>MRGSHHHHHHGSTEISLEGLHRNMGEQLFDGDILATGRIICRERHTGFHIQMNARQVEGRPGHYIVQGSKDTQSKLWVRLGREGWTSPTGGGQQGIVRSGQEEQVIFDVMADGNQWAKPGEYIFSVSGKCLTSWEDNKQNATAVA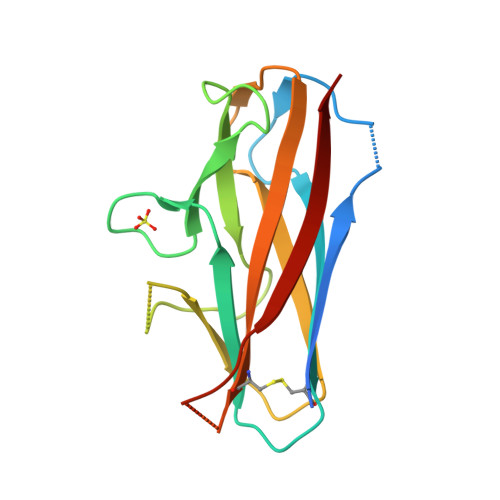KTATSTITVV[2x]>MGPMPKLADRKLCADQECSHPISMAVALQDYMAPDCRFLTIHRGQVVYVFSKLKGRGRLFWGGSVQG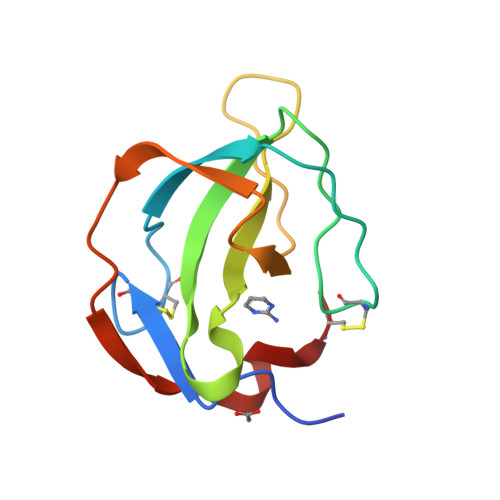DYYGDLAARLGYFPSSIVREDQTLKPGKVDVKTDKWDFYCQ[2x]Spr1654 is involved in the early steps of TA precursor synthesis, where the first amino sugar UDP-AATGal is suggested to be synthesized by this aminotransferase, followed by several TA biosynthesis pathway steps. The three-dimensional structures revealed that Spr1654 has a fold characteristic of the type I aminotransferase family. Each Spr1654 subunit can be divided into an N-terminal arm (residues 1–14), a large PLP-binding domain comprising residues 15–276 and a smaller C-terminal domain comprising residues 277–404. Two dimers, composed of subunits AB and CD, are present in the asymmetric unit of all the obtained crystals of all forms of Spr1654, with a buried surface area of 2490 Å2 per monomer (15% of the total solvent accessible surface area).

For Spr1654/PLP complex, 1 mM PLP was added into 1.5 mg ml−1 Spr1654, incubating at 20°C for 2 h, and the mixture was concentrated to 17.8 mg ml−1, by which excessive PLP was removed. In the crystal structure of the Spr1654/PLP complex, the PLP-binding sites are located at the bottom of deep and wide cavities formed at the interfaces between the subunits. The aromatic ring of PLP sits at the deep end of each cavity. Clear electron density confirms the formation of a covalent bond between PLP and residue Lys199 in Spr1654. Although the quality of the electron density is reduced in subunits C and D, the conformation of Lys199 confirms the presence of the internal aldimine in all subunits. The N1 atom of PLP is positioned at 2.8 and 3.2 Å from the OD1 and OD2 atoms of the conserved residue Asp170. These interactions enhance the electron sink nature of PLP and maintain the cofactor in a protonated state, which is a typical feature of the aspartate aminotransferase (AAT) type 1 enzyme family. The deprotonated O3′ of PLP is at a hydrogen-bond-forming distance from the side chain of residue His173, which preserves the negative charge of O3′, and stabilizes the protonated internal aldimine of Spr1654. The side chain of residue Tyr84 in Spr1654 forms van der Waals contact with the pyridine ring of PLP. In addition, the phosphate group forms two hydrogen bonds with the side chains of residues Ser194 and Thr59 in Spr1654, as well as water-mediated hydrogen bonds with the conserved residues Glu205 and Gly206.

>MASMTGMPNYNIPFSPPDITEAEITEVVDTLRSGWITTGPKTKELERRLSLYTQTPKTVCLNSATAALELILRVLEVGPGDEVIVPAMTYTASCSVITHVGATPVMVDIQADTFEMDYDLLEQAITEKTKVIIPVELAGIVCDYDRLFQVVEKKRDFFTASSKWQKAFNRIVIVSDSAHALGSTYKGQPSGSIADFTSFSFHAVKNFTTAEGGSATWKANPVIDDEEMYKEFQILSLHGQTKDALAKMQLGSWEYDIVTPAYKCNMTDIMASLGLVQLDRYPSLLQRRKDIVDRYDSGFAGSRIHPLAHKTETVESSRHLYITRVEGASLEERNLIIQELAKAGIASNVHYKPLPLLTAYKNLGFDMTNYPKAYAFFENEITLPLHTKLSDEEVDYIIETFKTVSEKVLTLSKKKLAAALEHHHHHH[4x]> PQSSQVTKRGLTDPERAAIIAAAVPDHALDTQRKYHYFIQPRWKRLSEYEQLSCYAQPNPDWIAGGLDWGDWTQKFHGGRPSWGNESTELRTTDWYRHRDPARRWHHPYVKDKSEEARYTQRFLAAYSSEGSIRTIDPYWRDEILNKYFGALLYSEYGLFNAHSSVGRDCLSDTIRQTAVFAALDKVDNAQMIQMERLFIAKLVPGFDASTDVPKKIWTTDPIYSGARATVQEIWQGV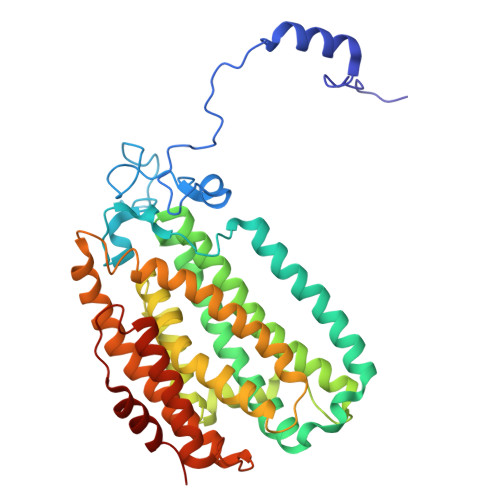QDWNEILWAGHAVYDATFGQFARREFFQRLATVYGDTLTPFFTAQSQTYFQTTRGAIDDLFVYCLANDSEFGAHNRTFLNAWTEHYLASSVAALKDFVGLYAKVEKVAGATDRAGVSEALQRVFGDWKIDYADKIGFRVDVDQKVDAVLAGYKN>[6x]MDHAPERFDATPPAGEPDRPALGVLELTSIARGITVADAALK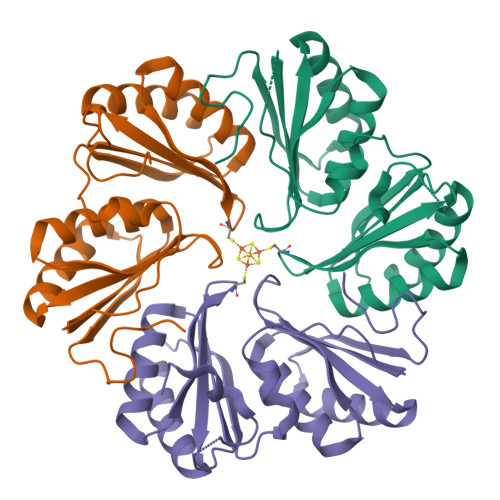RAPSLLLMSRPVCSGKHLLMMRGQVAEVEESMIAAREIAGAGSGALLDELELPYAHEQLWRFLDAPVVADAWEEDTESVIIVETATVCAAIDSADAALKTAPVVLRDMRLAIGIAGKAFFTLTGELADVEAAAEVVRERCGARLLELACIARPVDELRGRLFF Thiamine pyrophosphate (TPP) is the biologically active form of vitamin B1 (thiamine) and is essential for all living organisms. The same study also identified genes essential for growth on nutrient agar using high-density transposon mutagenesis, and found thiamine monophosphate kinase (ThiL) to be essential. In this study, we present high-resolution crystal structures of ThiL from the pathogen Acinetobacter baumannii (AbThiL) bound to substrate Thiamine monophosphate (TMP) and substrate analog adenylyl-imidodiphosphate (AMPPNP), and bound to its products TPP and adenosine diphosphate (ADP). The AbThiL structures assume the same two domain fold as MfThiL and AaThiLwith an N-terminal A domain and a C-terminal B domain.

Two crystal lattices were observed, an orthorhombic crystal form, and a monoclinic crystal form. Orthorhombic crystals were obtained from MCSG1 B1 (20% w/v PEG 4000, 600 mM NaCl, 100 mM MES/NaOH pH 6.5) and were harvested with reservoir with 20% v/v ethylene glycol, 5 mM ADP/TPP/MgCl2 added as cryo protectant. The orthorhombic crystal form was consistent for all complex structures and was refined for all ligands. For consistency, the orthorhombic ADP/TDP-bound structure will be used as the reference. The equivalent metal in the product complex is a magnesium ion as well, bridging between β-phosphate of TPP and β-phosphate in ADP and between α-phosphate and β-phosphate of ADP. In addition, we observed that the product complex (ADP/TPP) has a very similar conformation as the substrate complex. A superposition of the product complex and the substrate complex of AbThiL highlighs that the α-phosphate of TMP/TPP, and the α-phosphate and the β-phosphate groups of AMPPNP/ADP virtually do not move. Even the transferred phosphate group, the γ-phosphate in AMPPNP and the β-phosphate in TPP, barely changes position. The distance between the phosphorous atoms is only 1.0 Å.

>[2x]MAHHHHHHMAEFSIIDQYFNRQSHPDVALGIGDDSALITPPPNQQLVICADTLVAGRHFPLETSPHAIGWKSVAVNLSDIAAMGAKPHSILLAISLPQVDHEWLEGFSQGIYDCCNQFGVALIGGDTTQGPHLTITVTAMGWIETGKAVLRSGAKVGDYVCVSGQIGDAAYGLQHLGHSLQQRLDYPTPRCKLGEELKGLASSMIDVSDGLAQDLGHILKASKVGARLILEKLPVDPVLQQIEEQQRWQYALAGGDDYELCFTITPQNYEKLLQKQLDVKITMIGQIVEQTKLTFEHLGSDYPLQIHGYQHFA>[2x]MGRQWEEARALGRAVRMLQRLEEQCVDPRLSVSPPSLRDLLPRTAQLLREVAHSRREAGGGGPGGPGGSGDFLLIYLANLEAKSRQVA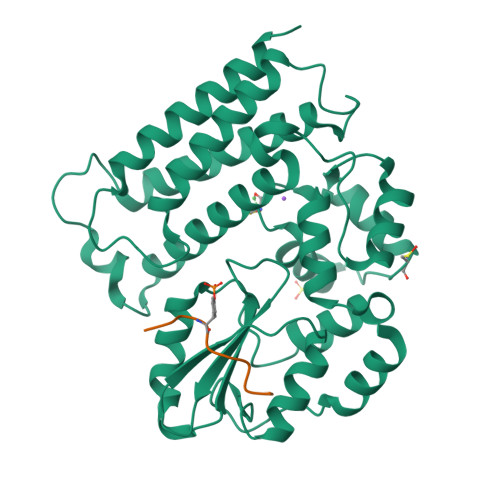ALLPPRGRRSANDELFRAGSRLRRQLAKLAIIFSHMHAELHALFPGGKYCGHMYQLTKAPAHTFWRESCGARCVLPWAEFESLLGTCHPVEPGCTALALRTTIDLTCSGHVSIFEFDVFTRLFQPWPTLLKNWQLLAVNHPGYMAFLTYDEVQERLQACRDKPGSYIFRPSCTRLGQWAIGYVSSDGSILQTIPANKPLSQVLLEGQKDGFYLYPDGKTHNPDLTELGAENLYFQ;>LQRYSSDPTGA[2x]4-oxobutanoic acid | C4 H6 O3 | 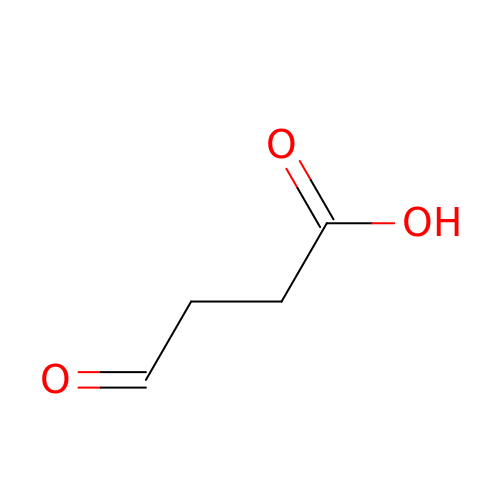UIUJIQZEACWQSV-UHFFFAOYSA-N> GSFTKKKGTITANVAGTKFEIVRLVIDEMGFMKTPDEDETSNLIWCDSAVQQEKISELQNYQRINHFPGMGEICRKDFLARNMTKMIKSRPLDYTFVPRTWIFPAEYTQFQNYVKELKKKRKQKTFIVKPANGAMGHGISLIRNGDKLPSQDHLIVQEYIEKPFLMEGYKFDLRIYILVTSCDPLKIFLYHDGLVRMGTEKYIPPNESNLTQLYMHLTNYSVNKHNEHFERDETENKGSKRSIKWFTEFLQANQHDVAKFWSDISELVVKTLIVAEPHVLHAYRMCRPGQPPGSESVCFEVLGFDILLDRKLKPWLLQINRAPSFGTDQKIDYDVKRGVLLNALKLLNIRTSDKRRNLAKQKAEAQRRLYGQNSIKRLLPGSSDWEQQRHQLERRKEEL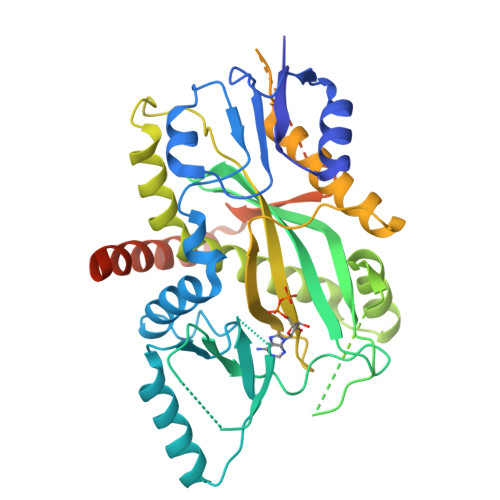KERLAQVRKQISREEHENRHMGNYRRIYPPEDKALLEKYENLLAVAFQTFLSGRAASFQRELNNPLKRMKEEDILDLLEQCEIDDEKL> SVDESKKRQWALEDFEIGRPLGKGKFGNVYLAREKQSKFILALKVLFKAQLEKAGVEHQLRREVEIQSHLRHPNILRLYGYFHDATRVYLILEYAPLGTVYRELQKLSKFDEQRTATYITELANALSYCHSKRVIHRDIKPENLLLGSAGELKIADFGWSVHAPSSRRTTLCGTLDYLPPEMIEGRMHDEKVDLWS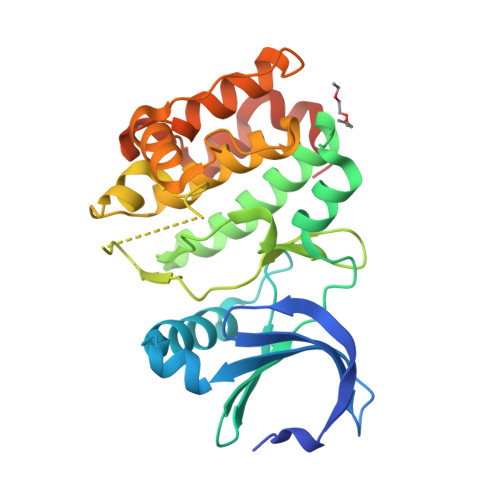LGVLCYEFLVGKPPFEANTYQETYKRISRVEFTFPDFVTEGARDLISRLLKHNPSQRPMLREVLEHPWITANSSKPSNCQNKESASKQS> MEKTTEGAFYTREYRNLFKEFGYSEAEIQERVKDTWEQLFGDNPETKIYYEVGDDLGYLLDTGNLDVRTAGMSYGMMMAVQMDRKDIFDRIWNWTMKNMYMTEGVHAGYFAWSCQPDGTKNSWGPAPDGEEYFALALFFASHRWGDGDEQPFNYSEQARKLLHTCVHNGEGGPGHPMWNRDNKLIKFIPEVEFSDPSYHLPHFYELFSLWANEEDRVFWKEAAEASREYLKIACHPETGLAPEYAYYDGTPNDEKGYGHFFSDSYRVAANIGLDAEWFGGSEWSAE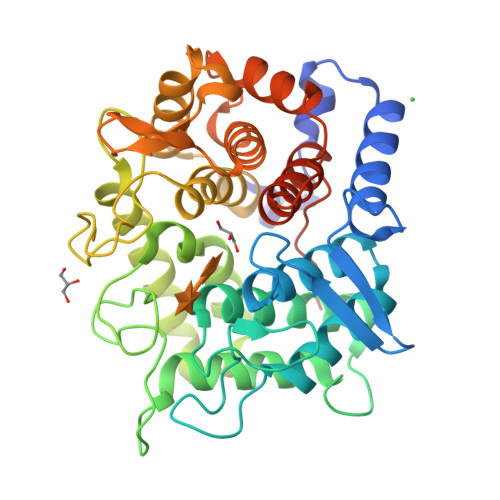EINKIQAFFADKEPEDYRRYKIDGEPFEEKSLHPVGLIATNAMGSLASVDGPYAKANVDLFWNTPVRTGNRRYYDNCLYLFAMLALSGNFKIWFPEGQEEEHLEHHHHHH> RQVIVPVCMPKIHYSPLKTGLCYDVRMRYHAKIFTSYFEYIDPHPEDPRRIYRIYKILAENGLINDPTLSGVDDLGDLMLKIPVRAATSEEILEVHTKEHLEFIESTEKMSREELLKETEKGDSVYFNNDSYASARLPCGGAIEACKAVVEGRVKNSLAVVRPPGHHAEPQAAGGFCLFSNVAVAAKNILK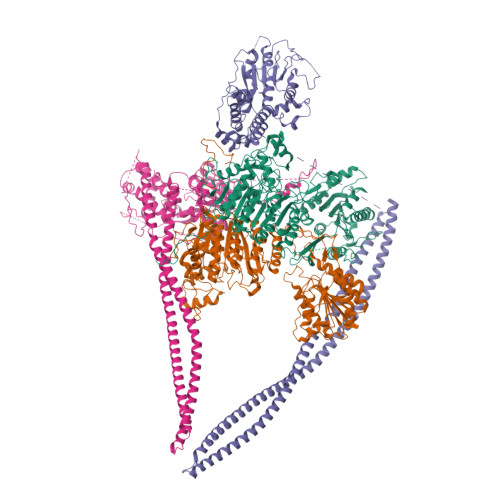NYPESVRRIMILDWDIHHGNGTQKSFYQDDQVLYVSLHRFEMGKYYPGTIQGQYDQTGEGKGEGFNCNITWPVGGVGDAEYMWAFEQVVMPMGREFKPDLVIISSGFDAADGDTIGQCHVTPSCYGHMTHMLKSLARGNLCVVLEGGYNLDAIARSALSVAKVLIGEPPDELPDPLSDPKPEVIEMIDKVIRLQSKYWNCFRRRHANSGCNFNEPINDSIISKNFPLQKAIRQQQQHYLSDEFNFVTLPLVSMDLPDNTVLCTPNISESNTIIIVVHDTSDIWAKRNVISGTIDLSSSVIIDNSLDFIKWGLDRKYGIIDVNIPLTLFEPDNYSGMITSQEVLIYLWDNYIKYFPSVAKIAFIGIGDSYSGIVHLLGHRDTRAVTKTVINFLGDKQLKPLVPLVDETLSEWYFKNSLIFSNNSHQCWKENESRKPRKKFGRVLRCDTDGLNNIIEERFEEATDFILDSFE;> ENSLSTTSKSKRQVIVPVCMPKIHYSPLKTGLCYDVRMRYHAKIFTSYFEYIDPHPEDPRRIYRIYKILAENGLINDPTLSGVDDLGDLMLKIPVRAATSEEILEVHTKEHLEFIESTEKMSREELLKETEKGDSVYFNNDSYASARLPCGGAIEACKAVVEGRVKNSLAVVRPPGHHAEPQAAGGFCLFSNVAVAAKNILKNYPESVRRIMILDWDIHHGNGTQKSFYQDDQVLYVSLHRFEMGKYYPGTIQGQYDQTGEGKGEGFNCNITWPVGGVGDAEYMWAFEQVVMPMGREFKPDLVIISSGFDAADGDTIGQCHVTPSCYGHMTHMLKSLARGNLCVVLEGGYNLDAIARSALSVAKVLIGEPPDELPDPLSDPKPEVIEMIDKVIRLQSKYWNCFRRRHANSGCNFNEPINDSIISKNFPLQKAIRQQQQHYLSDEFNFVTLPLVSMDLPDNTVLCTPNISESNTIIIVVHDTSDIWAKRNVISGTIDLSSSVIIDNSLDFIKWGLDRKYGIIDVNIPLTLFEPDNYSGMITSQEVLIYLWDNYIKYFPSVAKIAFIGIGDSYSGIVHLLGHRDTRAVTKTVINFLGDKQLKPLVPLVDETLSEWYFKNSLIFSNNSHQCWKENESRKPRKKFGRVLRCDTDGLNNIIEERFEEATDFILDSFE;> KVYYLPVTLTQFQKDLSEILISLHAKSFKASIIGEPQADAVNKPSGLPAGPETHPYPTLSQRQLTYIFDSNIRAIANHPSLLVDHYMPRQLLRMEPTESSIAGSHKFQVLNQLINSICFRDREGSPNEVIKCAIIAHSIKELDLLEGLILGKKFRTKRLSGTSLYNEKHKFPNLPTVDSTINKDGTPNSVSSTSSNSNSTSYTGYSKDDYDYSVKRNLKKRKINTDDWLFLATTKHLKHDQYLLANYDIDMIISFDPMLEVELPALQVLRNNANKDIPIIKLLVQNSPDHYLLDSEIKNSSVKSSHLSNNGHVDDSQEYEEIKSSLLYFLQARNAPVNNCEIDYIKLVKCCLEGKDCNNILPVLDLITLDEASKDSSDSGFWQPQLTKLQYSSTELPLWDGPLDIKTYQTELMHRAVIRLRDIQDEYAKGTVPLYEKRLNETQRQNQLDEIKNSVGLTFKKKQEVEKSINDSEKRLKHAMTESTKLQNKINHLLKNRQELENFNKLPSNTISSENHLEEGSALADKLKEYIDKNATLFNKLKELQQANAEKSKLNDELRSKYQIESSKAAESAQTLKILQESMKSLENEVNGPLTKFSTESLKKELERLQNDFQSLKARNKFLKNYITL;> SGDYWLPTTMSLYQKELTDQIVSLHYSDILRYFETSHYKEDVILESMKTMCLNGSLVATHPYLLIDHYMPKSLITRDVPAHLAENSGKFSVLRDLINLVQEYETETAIVCRPGRTMDLLEALLLGNKVHIKRYDGHSIKSKQKANDFSCTVHLFSSEGINFTKYPIKSKARFDMLICLDTTVDTSQKDIQYLLQYKRERKGLERYAPIVRLVAINSIDHCRLFFGKKFDKNSREYLENVTAAMVILRDRLGTLPPDLRPIYSQKLHYLVEWLENPTVPWPLPDIYPLKQYTSMDVERSLLTEVHFKKNSSNVNYHLSSGIITHKLIQSMGEVYMDICVQKQELDDYSCLDDLQNDHLKFFSNEDEKIIKEYETVLRTNNENLNRSHELEVENNLKFSQIETLEKDIETLKGSLMAQGETLSKLKDAFVKTDNVQDEIEKEERVSVSRDTEKKYMEQEIKRAVDAIRENEEETHKLNEKQNGLESELKLKFEKSEISTKELNEKIGFLKKELKLENDLNEELVGQLSKTMDNLENLTIPRVRTQ>[2x]EQWQTLYEAIGGEETVAKLVEAFYRRVAAHPDLRPIFPDDLTETAHKQKQFLTQYLGGPPLYTAEHGHPMLRARHLRFEITPKRAEAWLACMRAAMDEIGLSGPARE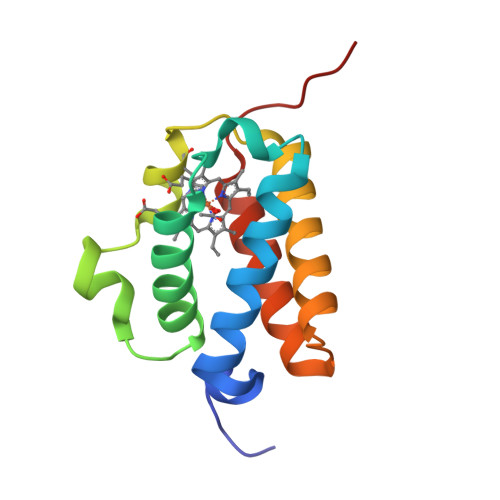QFYHRLVLTAHHMVNTPDHLD Cryptochromes (CRYs) are a structurally conserved but functionally diverse family of proteins that can confer unique sensory properties to organisms. In the marine bristle worm Platynereis dumerilii, its light receptive cryptochrome L-CRY (PdLCry) allows the animal to discriminate between sunlight and moonlight, an important requirement for synchronizing its lunar cycle-dependent mass spawning. The α-helical region contains the binding pocket for the major chromophore, flavin adenine dinucleotide (FAD), which is required for the light response. Here, we solve the structure of both dark state and blue light-illuminated PdLCry using cryo-electron microscopy (cryo-EM) in combination with single-particle reconstruction techniques.

The purified protein was vitrified in liquid ethane under far-red light conditions to produce cryo-EM grids of the dark state. We were able to refine the subset of particles composed of two subunits to obtain a dimeric structure with the PdLCry subunits arranged in parallel. As we did not observe any asymmetry during the reconstruction procedure, we enforced C2 symmetry in later reconstruction stages, yielding a final cryo-EM density map at 2.6 Å resolution. Our map shows an overall fold reminiscent of that observed in other type I CRYs, with an N-terminal α/β region (31-161) and a C-terminal α-helical region (243–524) connected by a largely well-resolved connector (162-242). The main dimer interface is formed between helices α8 of both subunits, with helices α8 running antiparallel at an angle of 42 degrees, flanked by interactions mediated by the connector region and the PBL. Apart from the differences in helix α8, we note unique dimer interactions involving Tyr266 of the PBL, especially with Pro279 (PBL) and Asn238 (connector) from the other subunit. A chain of four tryptophan residues, comprising TrpA428, TrpB405, TrpC351, and TrpD402, lines the path from the FAD to the protein surface and occupies identical positions as observed in the archetypical type I CRY DmCry. However, the sulfur loop of PdLCry has an additional surface-exposed Tyr352 that occupies a position similar to the terminal tyrosine in the type IV CRY ClCry4. In the dark state, the CTE is anchored in the vicinity of the FAD binding site by a CTT comprising residues 537 to 545.

>[2x]MKEKMSAWEVGNGIMEEKTDDWDNKEDNGKEHVSLHWFRHGLRLHDNPALLKSLEGAKEFYALFIWDGEVAGTKLVSYPRMKFLLECLKDLDDSLKKHGGRLYVVKGPSDVVIKQLIEEWGVTRVTCEIDPEPIWQPRDKAVKDLCATKGVKWFDYNSHLLWDPKAVCDANGGRPPHTYKLFCQVTDLLGKPETPHPDPDFSHVQMPVSDDFDDKFGLPTLKELGCEPECEEQEKPFNKWQGGETGALELLETRLMIERTAYKAGYIMPNQYIPDLVGPPRSMSPHLRFGALSIRKFYWDLHNNYAEVCGGEWLGALTAQLVWREYFYCMSYGNPSFDKMEGNPICLQIPWYKDEEALEKWKQGQTGFPWIDACMRQLRYEGWMHHVGRHAVACFLTRGDLWISWVDGLEAFYKYMLDGDWSVCAGNWMWVSSSAFENCLQCPQCFSPVLYGMRMDPTGEFTRRYVPQLKNMPLKYLFQPWKAPKEVQEKAGCVIGEDYPSPMVDHKEASSKCRRMMEDVKSIIKDPEVWHCTPSDTNEVRKFCWLPEHMTADQPCLGDLPCIKY> ALCCLW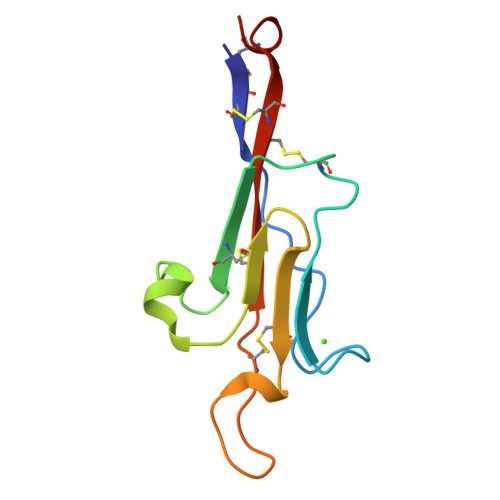SDWINEDHPSSGSDDGDRETFDGVCGAPEDIECRSVKDPHLSLEQLGQKVQCDVSVGFICKNEDQFGNGPFGLCYDYKIRVNCCWPMDKCA[2-oxidanylidene-7-[oxidanyl-[(1~{S})-1-phenylethyl]phosphoryl]oxy-chromen-4-yl]methanesulfonic 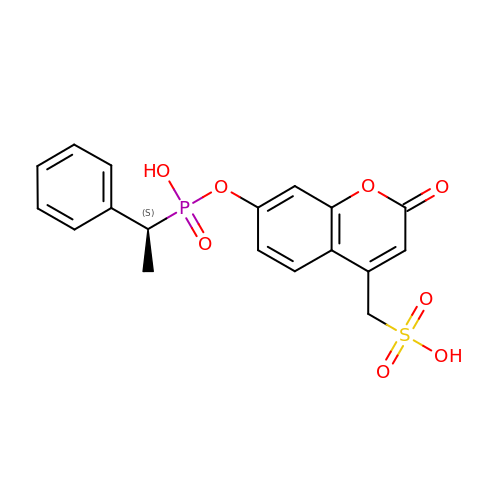acid | C18 H17 O8 P S | HLYLTMSHSJKDCP-LBPRGKRZSA-N>MKLKTTLFGNVYQFKDVKEVLAKANELRSGDVLAGVAAASSQERVAAKQVLSEMTVADIRNNPVIAYEDDCVTRLIQDDVNETAYNQIKNWSISELREYVLSDETSVDDIAFTRKGLTSEVVAAVAKICSNADLIYGAKKMPVIKKANTTIGIPGTFSARLQPNDTRDDVQSIAAQIYE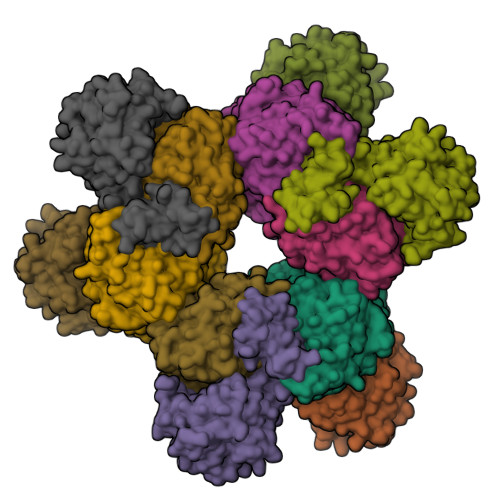GLSFGVGDAVIGVNPVTDDVENLSRVLDTIYGVIDKFNIPTQGCVLAHVTTQIEAIRRGAPGGLIFQSICGSEKGLKEFGVELAMLDEARAVGAEFNRIAGENCLYFETGQGSALSAGANFGADQVTMEARNYGLARHYDPFIVNTVVGFIGPEYLYNDRQIIRAGLEDHFMGKLSGISMGCDCCYTNHADADQNLNENLMILLATAGCNYIMGMPLGDDIMLNYQTTAFHDTATVRQLLNLRPSPEFERWLESMGIMANGRLTKRAGDPSLFF[2x];>[2x]MDQSSHHHHHHMDQKQIEEIVRSVMASMGQAAPAPSEAKCATTNCAAPVTSESCALDLGSAEAKAWIGVENPHRADVLTELRRSTVARVCTGRAGPRPRTQALLRFLADHSRSKDTVLKEVPEEWVKAQGLLEVRSEISDKNLYLTRPDMGRRLCAEAVEALKAQCVANPDVQVVISDGLSTDAITVNYEEILPPLMAGLKQAGLKVGTPFFVRYGRVKIEDQIGEILGAKVVILLVGERPGLGQSESLSCYAVYSPRMATTVEADRTCISNIHQGGTPPVEAAAVIVDLAKRMLEQKASGINMTR>[2x]GPGMAVKHLIVLKFKDEI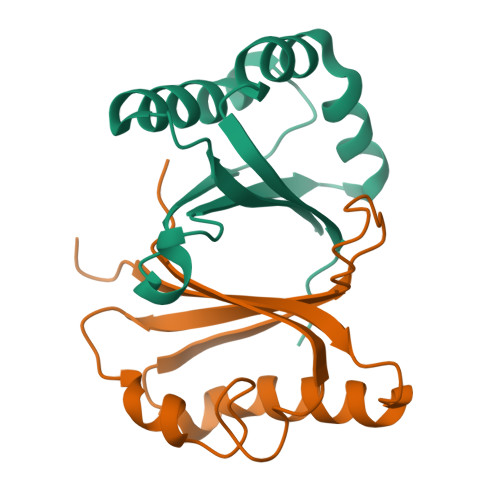TEAQKEEFFKTYVNLVNIIPAMKDVYWGKDVTQKNKEEGYTHIVEVTFESVETIQDYIIHPAHVGFGDVYRSFWEKLLIFDYTPRK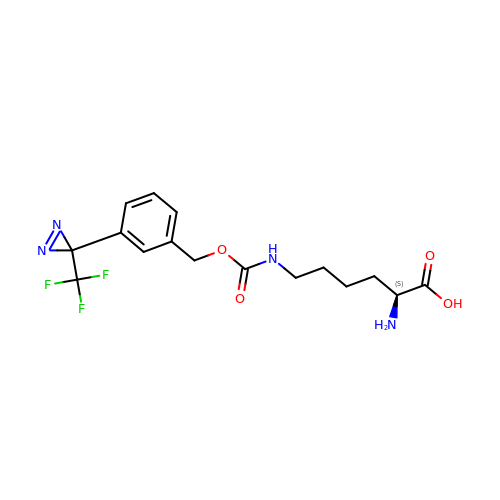N6-[({3-[3-(trifluoromethyl)-3H-diaziren-3-yl]phenyl}methoxy)carbonyl]-L-lysine | C16 H19 F3 N4 O4 | JHAONYPOHPLZAQ-LBPRGKRZSA-N> MSLSPHVENASIPKGSTPIPKNRNVSSIGKGEFLGSSSSNNSSFRMNHYSNSGQPSVLDSIRRPNLTPTFSYSNGVYMPESHRTSSFNDSYLPYDKNPYAKTTGSMSNKSNMKIKTKKNAINTNTRKSSGLIYTTKVDKELSSIDKVNDPNINGLVCAGKTHLGLYKFSPSDRSIKCVHDFITPNSNTSTRGTTSLLPKLSKRTRQNKFSTIADVKTGFNNYKNCIAVCNNSTAISIYDLNKSSSIDNPLITSLCEHTRSINSFDFNMVESNLIISGGQDSCVKIWDLRSNKSKSSNRSDISINTASDSIRDVKWMPGYNFASKNDQGSSTYGNLKSGYKFASIHDSGYLLKFDLRQPAQYEKKLNAHTGPGLCLNWHPNQEYIATGGRDGKCCLWFVGDNANAAENTVLNYGNSPSLHAPNTSLN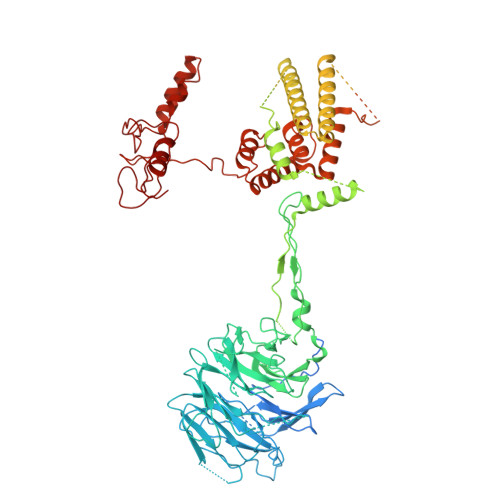NSGSLAFPKLTINTGYPVTKLKFKPAYSSNIYNSLLGISSMGDEAEVRIYSLARKYIPKHVLLSETPSLGLVWWDENLIFNIDKGTRINGWDINKEPTVLENLSKNTTTWRDLDGNGLLSVDQEIGSYEVVEPELQPTSSTTCKKHPGTIKNPKNGNPENQGIIGGIKKGFSHTGLTSFTPERPPTLKAGPTFSTKSLTLASGASSFNSSSASLTSLTPQTENREEIAIEPPCIITLDIPQIFNNIRLTKIAHSRKKNVISESSSMKNSPVEKFKYLARQLKFSYIREHNVSDSADTAYKNDIENIDVVKNATETHGDNTTTTNNNDDGDDDDDDDDDDKIIESHLLKKYNFPENNTWATLMNEKVNNKKSKRNSSSSREFDEKDVRSSISSISASRQSHDRARKIDKNVEAELQEKIQTLVDLISIATHNASVYLSIDDLTNFKIWILIRDSLLWDLKWMTSSQISSDNASNMDANESSDFEAGENLKTGKEFPEEDGAGTSGAESLVEERPQAFRANSDEPSDAEKKPVSKLKEQLKNTEIIPYAQPNEDSDEVLTKLKELQNQRLESRTKMGETVSDDVIIEEDEHEHQEEEQPHDSPTKSAQFHASPIAKSIPILQKREHRKSFIDTFMLHSPNGYNGDTDIGNEDDNISPRFTYNSVSPRSKVSSLQSYATTTSQLETFKKLSSHTAPIIGSPRHAPSRPDSIGREQLSSSLTKKLAKCKKIIADPPWDTKKLIKQLYNQATETGNVVLTVNILFLFQTIYQITEIDIAKDAIAHFLLLLHRYELFGIAADVLKYCPFEDIMGSEGDQSSIRLFCERCGELITNESSKEKLRAEAQQTGNKKIMDKFGYWYCDSCKKKNTSCVLCERPLKKLTMVILPCGHEGHFQCIQEWFLDENEQECPGGCPGVAFI>GHMQHPPRIAVIGAGPAGLTAALILHRGGHRVSVYEGEASGQQRTQGGTLDLHDDSGQVALQRAGLLEAFRAVARHEGQEARMGDPWSGEITTGGFGPEGSKDKPEIDRGDLRQLLLDALPADTVQWGHSLTALVSAQANGHGLRFANGVQREADIVIGADGAWSKVRAALSTCQPLPTGITFFEGWIAQPAADIAAMVGQGSLFCFGGEEALFVQRNSRDRLCVYAALKRSSEWLDAQIAQHGIRTLVTGCYTGWATNLRRLLEACTDFVRRPIYSLPADFCWTPRDGVTLIGDAAHLMPPVGVGVNLAMLDASDVAMALCARPDAISAMRDAEVLVRERARALMPDAIEGFQRWFITGGDAPRG[4x]

However, the genomes of several strains of this Gram-negative bacterium code for a FAD-dependent monooxygenase (SmTetX) homologous to tetracycline destructases. Activity assays using SmTetX showed its ability to modify oxytetracycline with a catalytic rate comparable to those of other destructases. SmTetX shares its fold with the tetracycline destructase TetX from Bacteroides thetaiotaomicron; however, its active site possesses an aromatic region that is unique in this enzyme family. The tetracycline destructases are classified as class A FAD-dependent monooxygenases (FDOs), which cover numerous proteins with diverse purposes and functions that primarily catalyze the hydroxylation of aromatic substrates.

Nevertheless, the structure of the protein could be solved using molecular replacement and refined at 1.95 Å resolution. The asymmetric unit consists of four SmTetX molecules with pairwise r.m.s.d.s on Cα atoms below 0.34 Å; the substrate-binding site remains structurally unchanged across the individual protein chains. There are two pairs of identical covalent dimers cross-linked via two disulfide bridges, i.e. chains A and B are linked via Cys172(A)–Cys172(B) and Cys281(A)–Cys281(B) disulfide bridges. The crystal structure contains SmTetX in the form of covalent dimers, which are most likely to be artefacts of crystallization. The enzyme shares its fold with the class A FAD-dependent monooxygenases. The overall structure of the monomer is divided into a smaller substrate-binding domain (residues Glu75–Ser99 and Pro176–Tyr274) and a larger FAD-binding domain (Met1–His74, Lys100–Leu175 and Ser275–Pro323), which are stabilized by a long C-terminal α-helix (Asp324–Arg364). FAD is observed in the IN conformation in our structure, i.e. FAD is elongated and its isoalloxazine moiety reaches into the re site. A chloride anion was modelled in the re site near the FAD isoalloxazine moiety according to the signal strength in the 2mF o − DF c map, the typical distances to adjacent atoms and their chemical properties. It is bound at the pyrimidine moiety of isoalloxazine and coordinated by the main-chain N atoms of the Pro300–Val303 loop.>GGACUCGGGGUGCCCUUCUGCGUGAAGGCUGAGAAAUACCCGUAUCACCUGAUCUGGAUAAUGCCAGCGUAGGGAAGU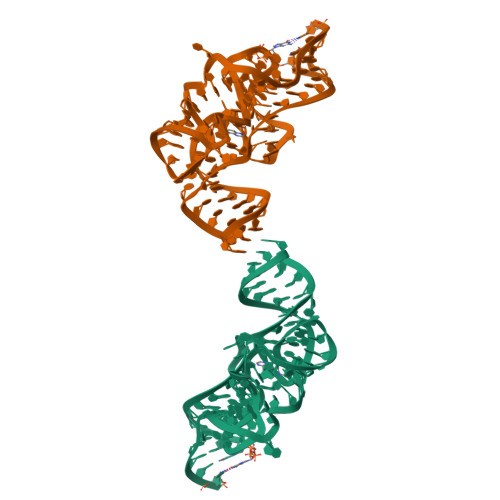UC[2x]>[2x]MLDEALMPKHIALIMDGNRRWAKDKGLDVSEGYKHLFPKLKEICDISSKLGIQVITAFAFSTENWKRAKGEVDFLMQMF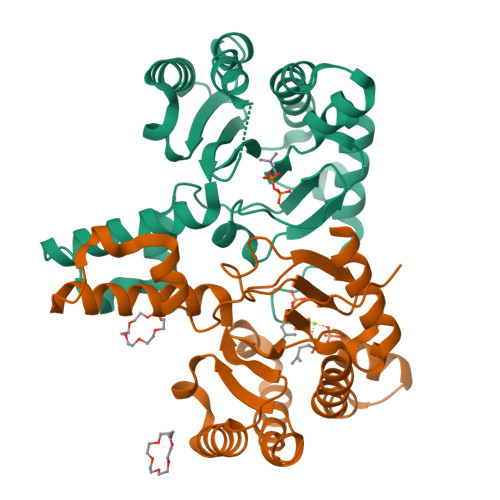EELYDEFSRSGVRVSIIGCKTDLPMTLQKCIALTEETTKGNKGLHLVIALNYGGYYDILQATKSIVNKAMNGLLDVEDINKNLFDQELESKCPNPDLLIRTGGDQRVSNFLLWQLAYTEFYFTKTLFPDFGEEDLKEAIINFQQRHRRFGGHTY> MGSQVSTQRSGSHENSNSATEGSTINYTTINYYKDSYAATAGKQSLKQDPDKFANPVKDIFTEMAAPLKSPSAEACGYSDRVAQLTIGNSTITTQEAANIIVGYGEWPSYCSDSDATAVDKPTRPDVSVNRFYTLDTKLWEKSSKGWYWKFPDVLTETGVFGQNAQFHYLYRSGFCIHVQCNASKFHQGAL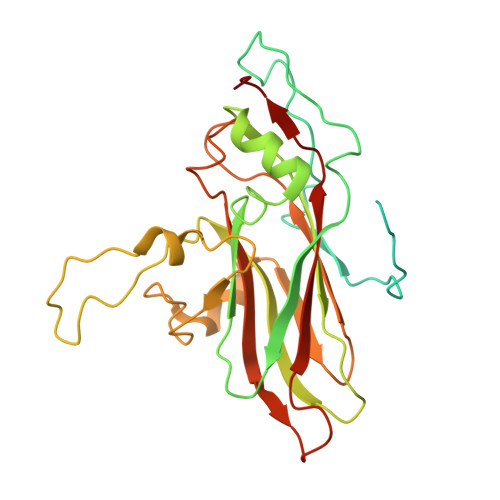LVAVLPEYVIGTVAGGTGTEDSHPPYKQTQPGADGFELQHPYVLDAGIPISQLTVCPHQWINLRTNNCATIIVPYINALPFDSALNHCNFGLLVVPISPLDYDQGATPVIPITITLAPMCSEFAGLRQAVTQ>[2x]SMQTTNIRKTFIFMEVLGSGAFSEVFLVKQRLTGKLFALKCIKKSPAFRDSSLENEIAVLKKIKHENIVTLEDIYESTTHYYLVMQLVSGGELFDRILERGVYTEKDASLVIQQVLSAVKYLHENGIVHRDLKPENLLYLTPEENSKIMITDFGLSKMEQNGIMSTACGTPGYVAPEVLAQK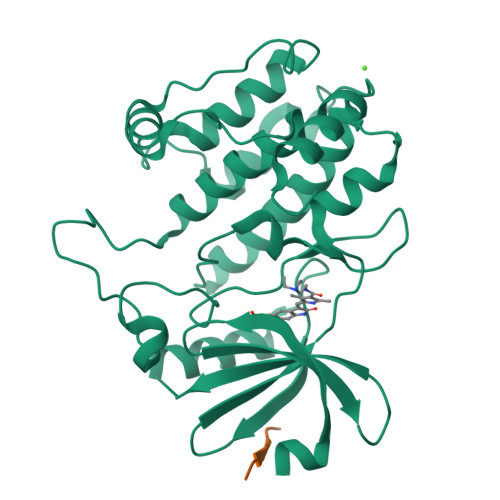PYSKAVDCWSIGVITYILLCGYPPFYEETESKLFEKIKEGYYEFESPFWDDISESAKDFICHLLEKDPNERYTCEKALSHPWIDGNTALHRDIYPSVSLQIQKNFAKSKWRQAFNAAAVVHH;> GVSKFA;> VSKF>[12x]MQGDPDVLKLLNEQLTSELT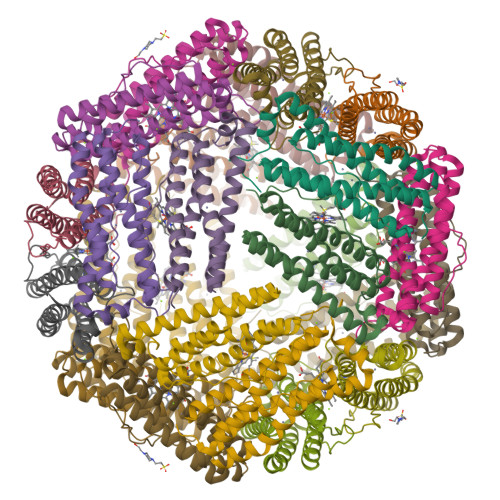AINQYFLHSKMQDNWGFTELAEHTRAESFEEMRHAETITDRILLLDGLPNYQRLFSLRVGQTLREQFEADLAIEYEVLERLKPGIVLCREKQDATSARLLEQILADEETHIDYLETQLQLMDKLGDALYAAQCVSRPPGSA> HHHHHHHMTAPAADDRIDEIERAITKSRRYQTVAPATVRR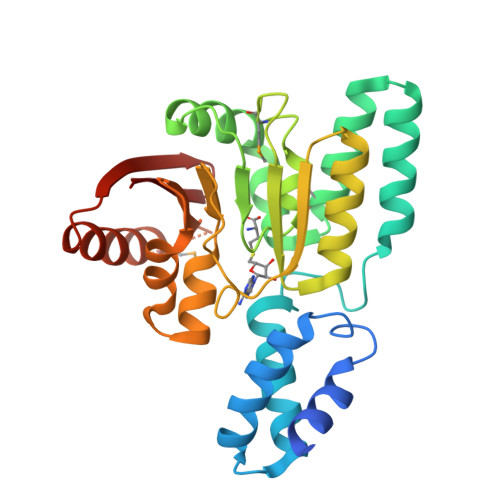LARAALVAARGDVPDAVKRTKRGLHEIYGAFLPPSPPNYAALLRHLDSAVDAGDDEAVRAALLRAMSVHISTRERLPHLDEFYRELFRHLPRPNTLRDLACGLNPLAAPWMGLPAETVYIASDIDARLVGFVDEALTRLNVPHRTNVADLLEDRLDEPADVTLLLKTLPCLETQQRGSGWEVIDIVNSPNIVVTFPTKSLGQRSKGMFQNYSQSFESQARERSCRIQRLEIGNELIYVIQK>[2x]PAARVEYIAPWWVVWLHSVPHLGLRLQRVDSTFSPGDETYQESLLFLGVLAAIGLGLNLIFLTVYLVCTCCCRRDHTVQTKQQESCCVTWTAVVAGLLCCAAVGVGFYGNSETNDGMHQLIYSLDNANHTFSGMDELVSANTQRMKVDLEQHLARLSEIIAARGDYIQTLKFMQQMAGNVVSQLSGLPVWREVTTQLTKLSHQTAYVEYYRWLSYLLLFILDLVICLVTCLGLARRSKCLLASMLCCGILTLILSWASLAADAAAAVGTSDFCMAPDIYILNNTGSQINSEVTRYYLHCSQSLISPFQQSLTTFQRSLTTMQIQVGGLLQFAVPLFPTAEKDLLGIQLLLNNSEISLHQLTAMLDCRGLHKDYLDALTGICYDGIEGLLFLGLFSLLAALAFSTLTCAGPRAWKYFINRDRDYDDIDDDDPFNPQARRIAAHNPTRGQLHSF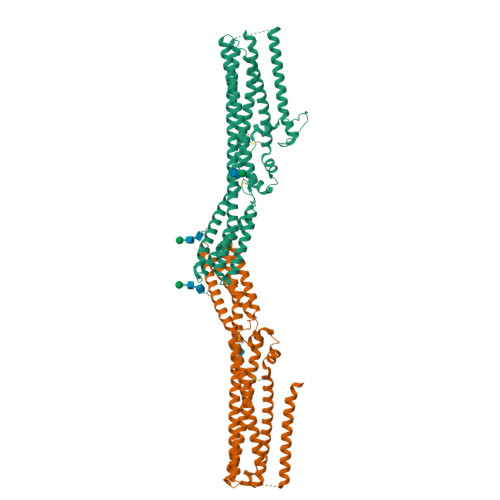CSYSSGLGSQCSLQPPSQTISNAPVSEYMNQAILFGGNPRYENVPLIGRGSPPPTYSPSMRPTYMSVADEHLRHYEFPSSNSLEVLFQ>YKQCHKKGGHCFPKEKICLPPSSDFGKMDCRWRWKCCKKGSG[3x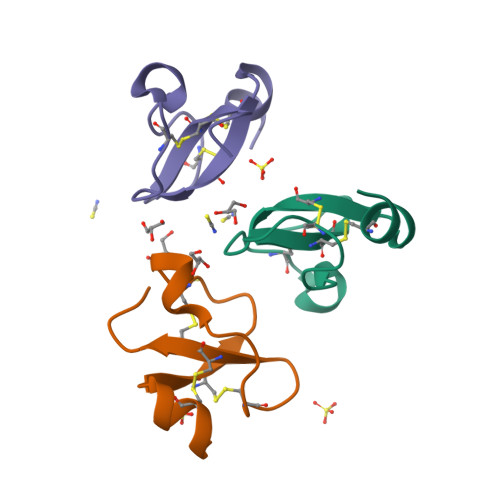]>GSHMDINNKARIHWACRRGMRELDISIMPFFEHEYDSLSDDEKRIFIRLLECDDPDLFNWLMNHGKPADAELEMMVRLIQTRNRERGPVAI[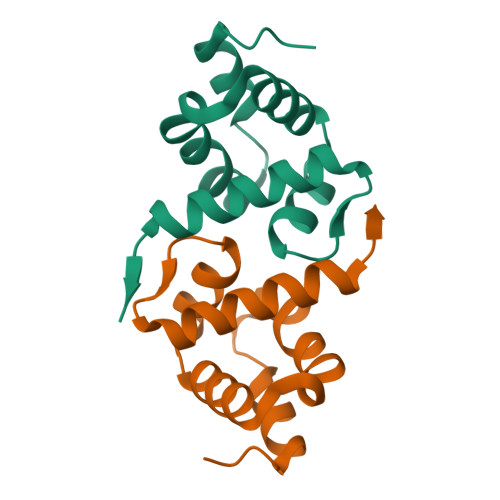2x]>GSGERKISRIHLVSEPSITHFLQVSWEKTLKSGFVITLTDGHSAWTGTVSESKISQEAATMAMNKGKYVGELRKALLSGAGPADVYTFNFSKESRYFFFKKNLKDVSFRLGSFNLEKVENPAE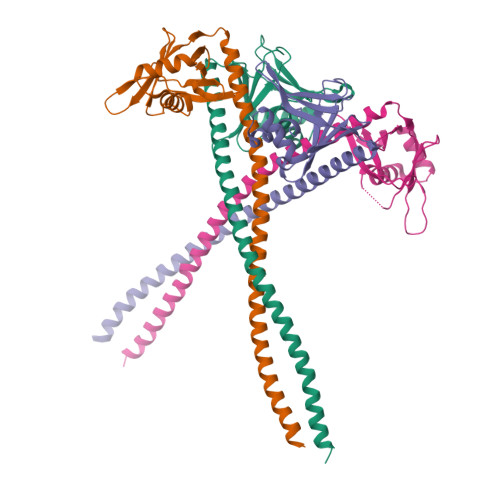VIRELIDYALDRNNLLQAELEELRAVVEQTERSRKLAEQELIETSERVQLLHSQNTSLINQKKKMDADLSQLQTEVEEAVQECRNAEEKAKKA[4x]> GSAEDKSKRDSIGLNAKEGQTNNGFVQNEDILETDLDPSSPAAGPQHNTVDILGPGEPDVKDVRPYAGMPKEVLFQFSGQARYRIPREVLFWLTVASVLLLIAATIAIIAISPKCLDWWQAGPMYQIYPRSFRDSNKDGDGDLKGIQDKLDYITTLNIKTVWITSFYKSSLKDFRHAVEDFQEIDPIFGTMKDFENLVAAIHDKGLKLIIDFIPNHTSDKHAWFQWSRNRTGKYTDYYIWHDCNYENGTTIPPNNWLSVYGNSSWHFDEVRKQCYFHQFMKEQPDLNFRNPDVQEEIKEIIQFWLSKGVDGFSFNALQYLLEAKHLRDEAQVNKTQIPDTVTHYSQLHHDFTTTQVGMHDIVRSFRQTMNQYSREPGRYRFMGTEAHGESITETMVYYGLPFIQEADFPFNSYLSKLDKPSGNSVSEVITSWLENMPEGKWPNWMTGGPDNVRLTSRLGEKYVNIMNMLVFTLPGTPITYYGEEIGMRNILAANLNENYDTGTLFSKSPMQWDNSSNAGFSEGNHTWLPTSSDYHTVNVDVQKTQPRSALKLYQELSLLHANELLLSRGWFCYLRNDNHSIMYTRELDGINKVFLMVLNFGESSLLNLKEMISNIPTRVRIRLSTSSAYSGREVDTHAVTLASGEGLILEYNTGNLLHRQTAFKDRCFVSNRACYSRVLNILYSLC

Cystinuria is caused by mutations in system b0,+, which is a Na+-independent cystine/dibasic amino acid exchanger localized at brush border cells in the kidney and intestine. Mutations of the regulatory glycoprotein rBAT and the amino acid transporter b0,+AT, which constitute system b0,+, are linked to type I and non-type I cystinuria respectively and they exhibit distinct phenotypes due to protein trafficking defects or catalytic inactivation. Here, using electron cryo-microscopy and biochemistry, we discover that Ca2+ mediates higher-order assembly of system b0,+. Ca2+ stabilizes the interface between two rBAT molecules, leading to super-dimerization of b0,+AT–rBAT, which in turn facilitates N-glycan maturation and protein trafficking.

To further improve the map quality, we performed the multi-body refinement and focused refinement, improving the map resolution to 2.6 Å for the extracellular domain and 3.0 Å for the individual heterodimer. The ectodomain displays a glucosidase-like fold, which consists of domains A, B, and C. The domain B is unique to rBAT (not present in CD98hc) and composed of two insertion loops within domain A. For simplicity, we refer to the first loop as domain B-I (residues 213–289) and the second loop as domain B-II (residues 318–355). Domain B-II interacts with the adjacent rBAT molecule and thereby contributes to the formation of higher-order assemblies. The interaction involves six salt bridges, one π-cation-π stacking and several hydrophobic interactions, which together give rise to the strong higher-order assembly. The cryo-EM map of rBAT revealed a strong spherical density in the middle of domain B. This density is surrounded by the acidic side chains of Asn214′, Asp284′ and Glu321′ and the main chain carbonyl groups of Tyr318′ and Leu319′, indicative of a metal cation. In rBAT, the Ca2+ ion bridges domains B-I and B-II to reinforce the super-dimer interface. Electrostatic potential calculations of rBAT with or without Ca2+ showed that Ca2+ neutralizes the super-dimer interface to facilitate the homomeric interaction.> GVGRVAFVFPGQGTQWAGMGAELLDSSAVFAAAMAECEAALSPYVDWSLEAVVRQAP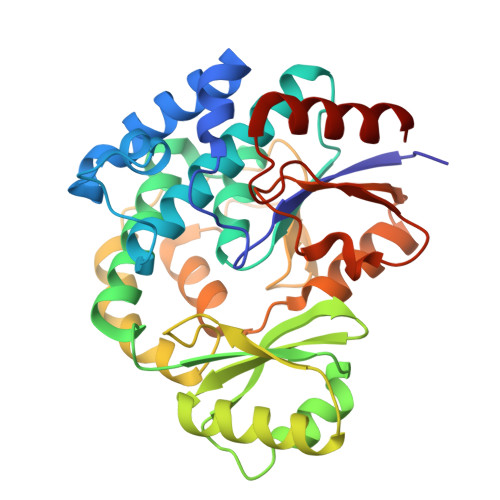GAPTLERVDVVQPVTFAVMVSLARVWQHHGVTPQAVVGHSQGEIAAAYVAGALSLDDAARVVTLRSKSIAAHLAGKGGMLSLALSEDAVLERLAGFDGLSVAAVNGPTATVVSGDPVQIEELARACEADGVRARVIPVDYASHSRQVEIIESELAEVLAGLSPQAPRVPFFSTLEGAWITEPVLDGGYWYRNLRHRVGFAPAVETLATDEGFTHFVEVSAHPVLTMALPGTVTGLATLRRDNGGQDRLVASLAEAWAN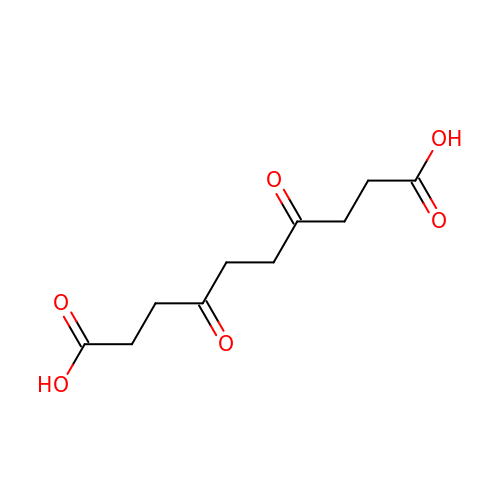4,7-DIOXOSEBACIC ACID | C10 H14 O6 | DUAWJQCMZICMIK-UHFFFAOYSA-N>[2x]GPGGEMQKIVFKIPMVDDKSRTKAM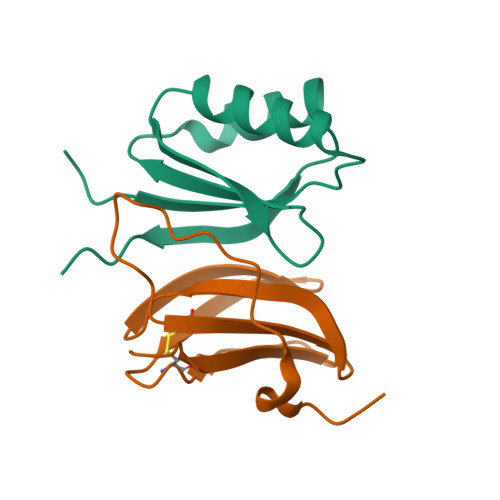SLVASTVGVHSVAIAGDLRDQVVVVGDGIDSINLVSALRKKVGPAMFLEVSQVKED;>METGNKYIEKRAIDLSRERDPNFFDHPGIPVPECFWFMFKNNVRQDAGTCYSSWKMDMKVGPNWVHIKSDDNCNLSGDFPPGWIVLGKKRPGF[2x]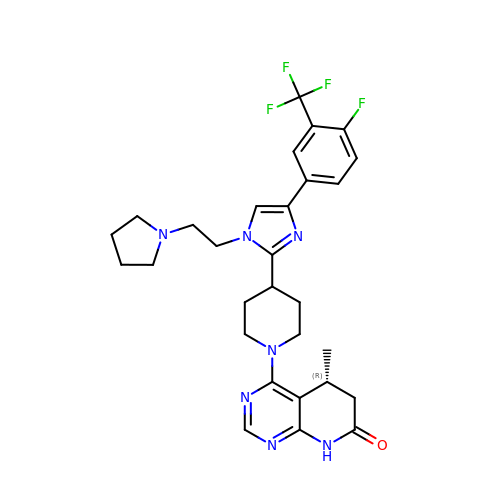(5R)-4-(4-{4-[4-fluoro-3-(trifluoromethyl)phenyl]-1-[2-(pyrrolidin-1-yl)ethyl]-1H-imidazol-2-yl}piperidin-1-yl)-5-methyl-5,8-dihydropyrido[2,3-d]pyrimidin-7(6H)-one | C29 H33 F4 N7 O | XIYKGCYSJCRNDN-GOSISDBHSA-N We focus on AMGs that potentially encode chitosanase enzymes that metabolize chitin – a common carbon polymer. One expressed protein showing endo-chitosanase activity (V-Csn) is crystalized and structurally characterized at ultra-high resolution, thus representing the structure of a soil viral AMG product. The structure consisted of two non-contiguous structural domains. Our rigorous analyses not only resulted in a crystal structure of a soil viral AMG product, but also enabled us to propose the mode of action of this previously uncharacterized chitosanase enzyme in the GH75 family of glycosyl hydrolases.

The V-Csn structure was solved in two crystal forms; apo1 containing a single molecule in the asymmetric unit, and apo2 containing a dimer in the asymmetric unit. The apo1 structure was solved by single anomalous diffraction (SAD) methods using the signal from bromide ions soaked into crystals of the apo1 form. Refinement was completed with phenix.refine24 against a high resolution apo1 data set extending to 0.89 Å resolution. The final model comprised 1811 protein atoms in a single chain, 398 water molecules, three glycerol and a sulfate anion. The final Rwork and Rfree were 0.1198 and 0.1307 for 174,427 total reflections. A single V-Csn molecule was located in the apo1 asymmetric unit. The N-terminal part of Domain-1 (residues 1-36) is folded first and the polypeptide then folds the entire Domain-2 (residues 37-108) before crossing back to complete Domain-1 (residues 109-224). Inspection of the apo1 structure shows that the two residues identified as putative active site residues (D148 and E157) are located in a cleft between the two structural domains. Two additional acidic residues (D34 and D36) are also located in this cleft adjacent to D148, and these residues were also conserved in the other GH75 chitosanases. In V-Csn, the side chain of D148 makes hydrogen bonding interactions with the main chain amide nitrogen of A92 and the side chains of both D34 and D36.

> GSHMSELSEIDSVAGVTIYSVDGEPKSFVYKAGFAIDADGAPNAYAPNNGGTDFTANGGDDQGGDWWGGPVDAEGYPIKQKIFDPFPGYYVSATAHFNPAYSEDSPYRYIDSNSIPFIVLPGNHSNGAKLGDVALVYNEKTGDNCYAIYGDVGPSSKIGEGSVRLAQALKIDDNPKAGGTESRIVVTLVFPGSVGKWETPKRWFSHANQLTKAWGGLSRLKTLSDQL>[2x]MPSFDIVSEITLHEVRNAVENANRVLSTRYDFRGVEAVIELNEKNETIKITTESDFQLEQLIEILIGSCIKRGIEHSSLDIPAESEHHGKLYSKEIKLKQGIETEMAKKI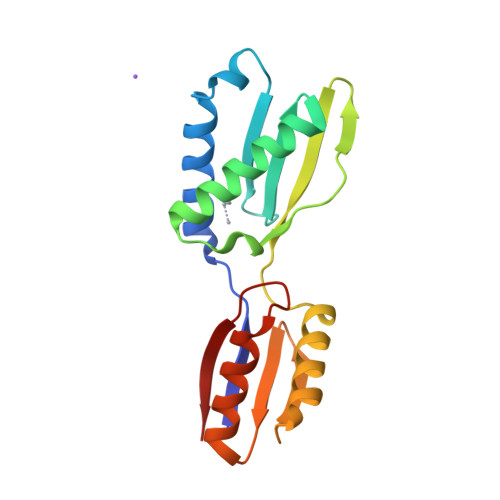TKLVKDSKIKVQTQIQGEQVRVTGKSRDDLQAVIQLVKSAELGQPFQFNNFRD>[2x]MNPIQLDTLLSIIDEGSFEGASLALSISPSAVSQRVKALEHHVGRVLVSRTQPAKATEAGEVLVQAARKMVLLQAETKAQLSGRLAEIPLTIAINADSLSTWFPPVFNEVASWGGATLTLRLEDEAHTLSLLRRGDVLGAVTREANPVAGCEVVELGTMRHLAIATPSLRDAYMVDGKLDWAAMPVLRFGP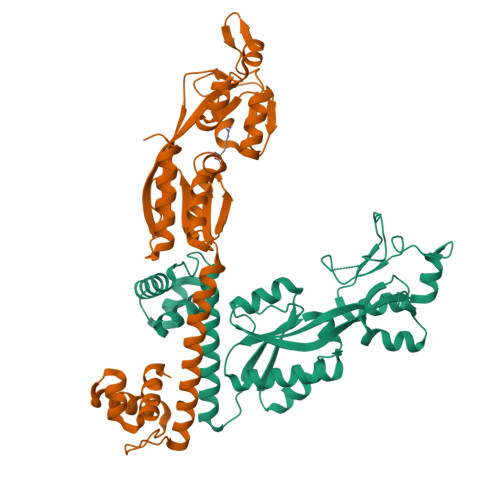KDVLQDRDLDGRVDGPVGRRRVSIVPSAEGFGEAIRRGLGWGLLPETQAAPMLKAGEVILLDEIPIDTPMYWQRWRLESRSLARLTDAVVDAAIEGLRP>[8x]MSAKKIVLKSSDGESFEVEEAV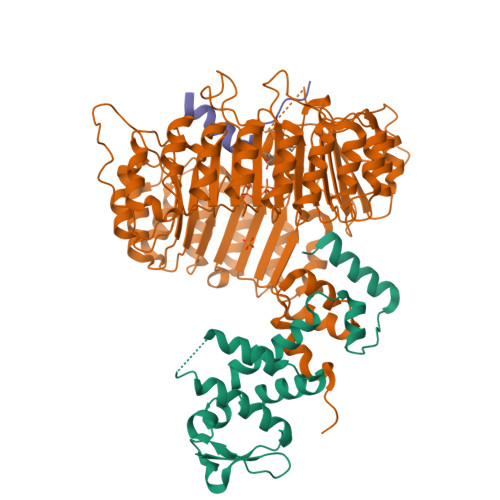ALESQTIAHMVEDDCVDNGVPLPNVTSKILAKVIEYCKRHVEAAASKAEAVEGAATSDDDLKAWDADFMKIDQATLFELILAANYLNIKNLLDLTCQTVADMIKGKTPEEIRTTFNIKNDFTPEEEEEVRRENQWAFE;>MEDPDIKRCKLSCVATVDDVIEQVMTYITDPKDRDSASLVCRRWFKIDSETREHVTMALCYTATPDRLSRRFPNLRSLKLKGKPRAAMFNLIPENWGGYVTPWVTEISNNLRQLKSVHFRRMIVSDLDLDRLAKARADDLETLKLDKCSGFTTDGLLSIVTHCRKIKTLLMEESSFSEKDGKWLHELAQHNTSLEVLNFYMTEFAKISPKDLETIARNCRSLVSVKVGDFEILELVGFFKAAANLEEFCGGSLNEDIGMPEKYMNLVFPRKLCRLGLSYMGPNEMPILFPFAAQIRKLDLLYALLETEDHCTLIQKCPNLEVLETRNVIGDRGLEVLAQYCKQLKRLRIERGADEQGMEDEEGLVSQRGLIALAQGCQELEYMAVYVSDITNESLESIGTYLKNLCDFRLVLLDREERITDLPLDNGVRSLLIGCKKLRRFAFYLRQGGLTDLGLSYIGQYSPNVRWMLLGYVGESDEGLMEFSRGCPNLQKLEMRGCCFSERAIAAAVTKLPSLRYLWVQGYRASMTGQDLMQMARPYWNIELIPSRRVPEVNQQGEIREMEHPAHILAYYSLAGQRTDCPTTVRVLKEPI[8x];>ELPIARRASLHRFLEKRKDRV[7x]>MNPQTDNVFYATNAFTGEALPLAFPVHTEVEVNQAATAAAKVARDFRRLNNSKRASLLRTIASELEARSDDIIARAHLETALPEVRLTGEIARTANQLRLFADVVNSGSYHQAILDTPNPTRAPLPKPDIRRQQIALGPVAVFGASNFPLAFSAAGGDTASALAAGCPVIVKGHTAHPGTSQIVAECIEQALKQEQLPQAI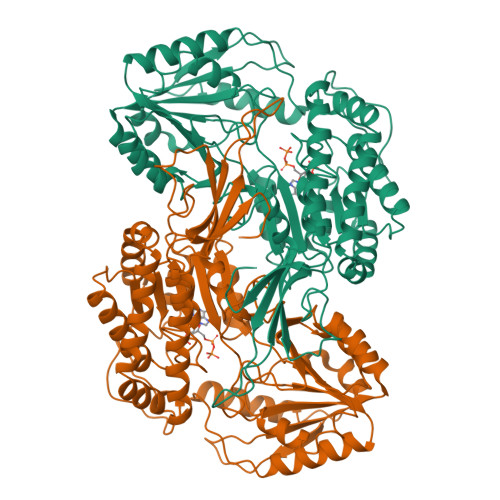FTLLQGNQRALGQALVSHPEIKAVGFTGSVGGGRALFNLAHERPEPIPFYGELGAINPTFIFPSAMRAKADLADQFVASMTMGCGQFCTKPGVVFALNTPETQAFIETAQSLIRQQSPSTLLTPGIRDSYQSQVVSRGSDDGIDVTFSQAESPCVASALFVTSSENWRKHPAWEEEIFGPQSLIVVCENVADMLSLSEMLAGSLTATIHATEEDYPQVSQLIPRLEEIAGRLVFNGWPTGVEVGYAMVHGGPYPASTHSASTSVGAEAIHRWLRPVAYQALPESLLPDSLKAENPLEIARAVDGKAAHS[4x]> GPLGSPEFDCHLSDMLQQLHSVNASKPSERGLVRQEEAEDPACIPIFWVSKWVDYSDKYGLGYQLCDNSVGVLFNDSTRLILYNDGDSLQYIERDGTESYLTVSSHPNSLMKKITLLKYFRNYMSEHLLKAGANITPREGDELARLPYLRTWFR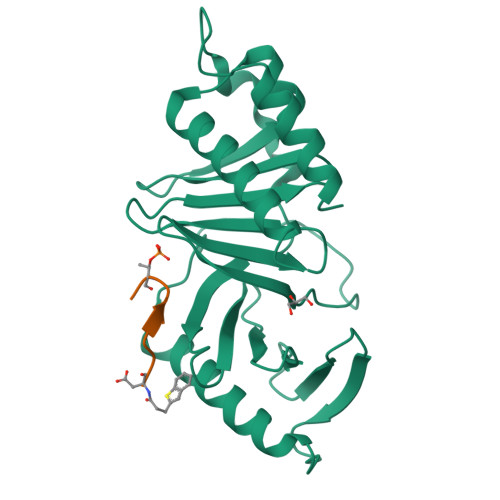TRSAIILHLSNGSVQINFFQDHTKLILCPLMAAVTYIDEKRDFRTYRLSLLEEYGCCKELASRLRYARTMVDKLLSSR;> XDPPLHSTAX>[4x]GVSDIQEAVAQIKAAGPSKPRLARDPVNQPMINNWVEAIGDRNPIYVDDAAARAAGHPGIVAPPAMIQVWTMMGLGGVRPKDDPLGPIIKLFDDAGYIGVVATNCEQTYHRYLLPGEQVSISAELGDVVGPKQTALGEGWFINQHIVWQVGDEDVAEMNWRILKFKPAGSPSSVPDDL;>[4x]MTVVGAVLPELKLYGDPTFIVSTALATRDFQDVHHDRDKAVAQGSKDIFVNILTDT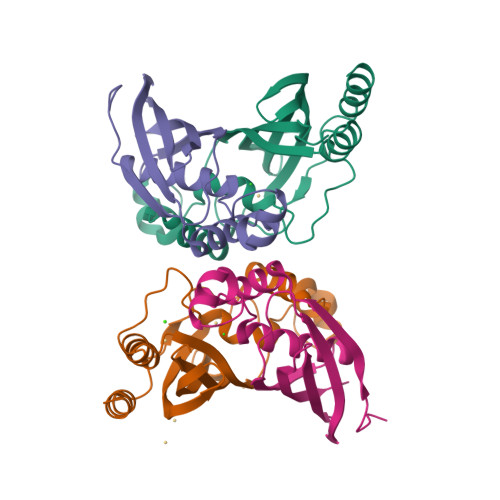GLVQRYVTDWAGPSALIKSIGLRLGVPWYAYDTVTFSGEVTAVNDGLITVKVVGRNTLGDHVTATVELSMR>[2x]SLFELGKMILQETGKNPAKSYGAYGC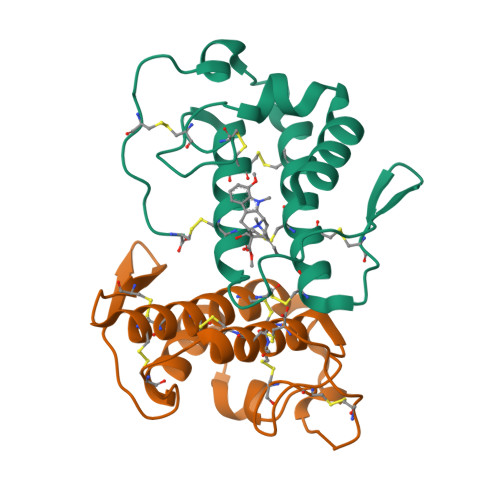NCGVLGRGKPKDATDRCCYVHKCCYKKLTGCDPKKDRYSYSWKDKTIVCGENNPCLKELCECDKAVAICLRENLGTYNKKYRYHLKPFCKKADPC> MGIGIYSPGIWRIPHLEKFLAQPCQKLSLLRPVPQEVNAIAVWGHRPSAAKPVAIAKAAGKPVIRL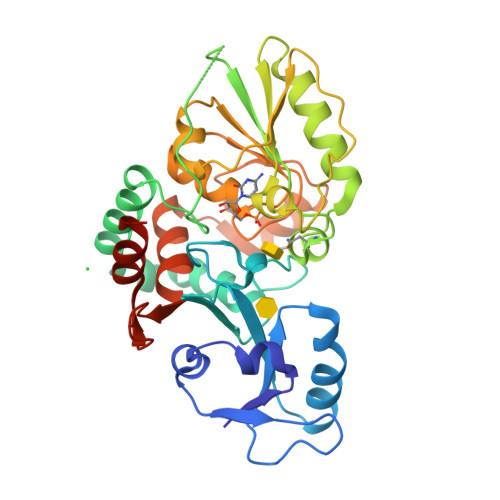EDGFVRSLDLGVNGEPPLSLVVDDCGIYYDASKPSALEKLVQDKAGNTALISQAREAMHTIVTGDMSKYNLAPAFVADESERTNIVLVVDQTFNNMSVTYGNAGPHEFAAMLEAAMAENPQAEIWVKVHPDVLEGKKTGYFADLRATQRVRLIAENVSPQSLLRHVSRVYVVTSQYGFEALLAGKPVTCFGQPWYASWGLTDDRHPQSALLSARRGSATLEELFAAAYLRYCRYIDPQTGEVSDLFTVLQWLQLQRRHHHHHH>CACCNAGCG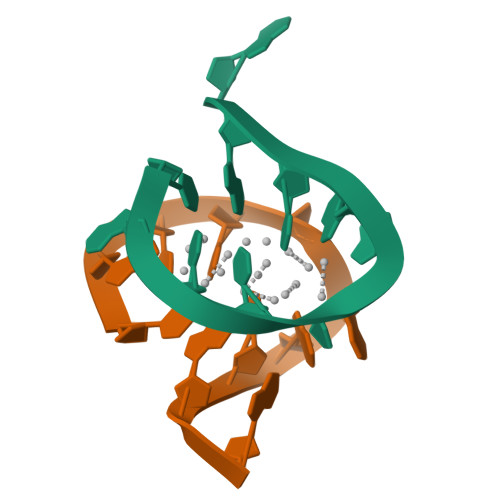A[2x]>GSHHHDPLTGLPNRLLFESRLNHALDEAREESRPGAVLFIDLDRFKHINDSLGHPIGDLLLKAIAERLRDQLRDVDTVARLGGDEFIILLPGLHQESDAEHVARKLLNAFTAPFQADGHEFFVSASVGIALFPKDGDDAPTLVKNADAAMYRAKSRGRSRIEYYTRELTYLATERMALETELRRALERDELQLYYQPKLSLESGLLVGAEALVRWYHPLFGEISPERFIPLAEDCGLILPLGDWVLEHACQQMGEWQKLHAPFGPLSVNLAGAQLGQPQLIERLEQLLEQSGLEPSRLQLEITESFIMNQTEEALAVLHGLKRLGVQLAIDDFGTGYSSLSYLKRLPLDILKIDKSFIRGLPDDPHD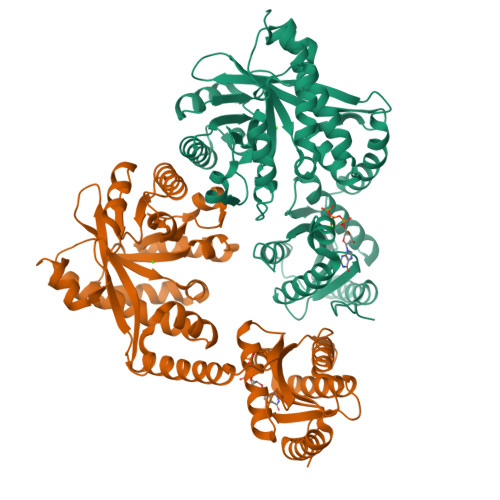AAITRAIIALGRSMQLTVIAEGVETEGQQSFLTHEGCEQIQGFVLSPPLPAELFASKFLKPRQPIGAPREAPV[2x]> DALHDQASALFKPIPEQVTELRGQPISEQQRELGKKLFFDPRLSRSHVLSCNTCHNVGTGGADNVPTSVGHGWQKGPRNSPTVFNAVFNAAQFWDGRAKDLGEQAKGPIQNSVEMHSTPQLVEQTLGSIPEYVDAFRKAFPKAGKPVSFDNMALAIEAYEATLVTPDSPFDLYLKGDDKALDAQQKKGLKAFM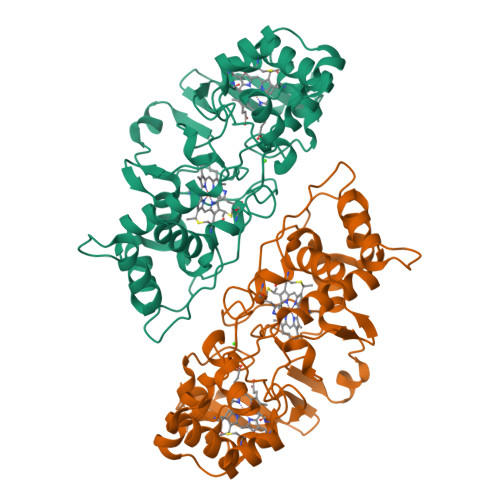DSGCSACHNGINLGGQAYFPFGLVKKPDASVLPSGDKGRFAVTKTQSDEYVFRAAPLRNVALTAPYFHSGQVWELKDAVAIMGNAQLGKQLAPDDVENIVAFLHSLSGKQPRVEYPLLPASTETTPRPAE> RLSLQNTAEIQHCLVNAGDVGCGVFECFENNSCEIRGLHGICMTFLHNAGKFDAQGKSFIKDALKCKAHALRHRFGCISRKCPAIRE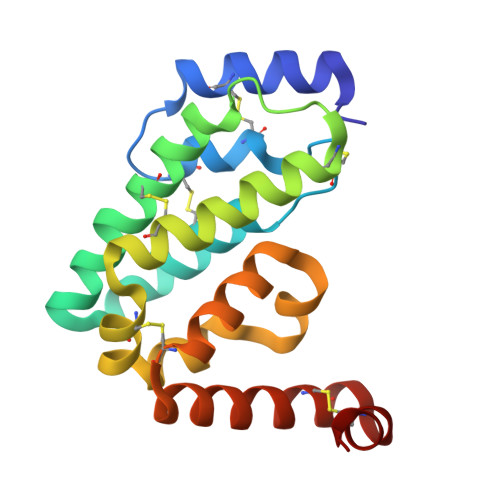MVSQLQRECYLKHDLCAAAQENTRVIVEMIHFKDLLLHEPYVDLVNLLLTCGEEVKEAITHSVQVQCEQNWGSLCSILSF ethyl (2R,4S)-4-{[3,5-bis(trifluoromethyl)benzyl](methoxycarbonyl)amino}-2-ethyl-6-(trifluoromethyl)-3,4-dihydroquinoline-1(2H)-carboxylate | C26 H25 F9 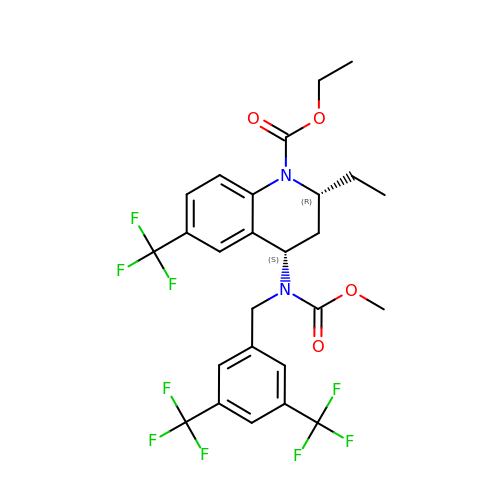N2 O4 | CMSGWTNRGKRWGS-NQIIRXRSSA-N>[3x]MAHHHHHHMSHCLIAPSIL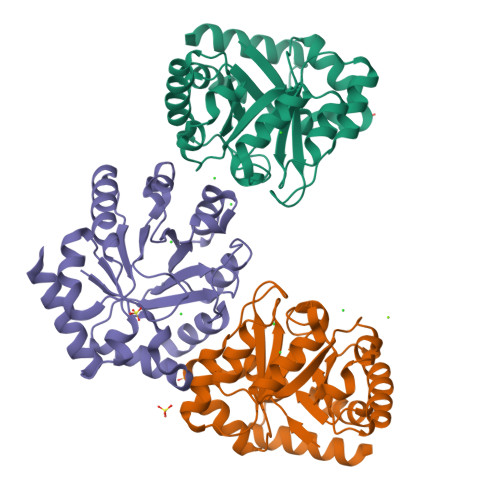SANFARLGEEVDNVLAAGADWVHFDVMDNHYVPNLTIGPMVCQALRKHGVTAPIDVHLMVEPVDRIIPDFAEAGATYISFHPEASRHVHRTIQLIRSLGCKPGIVLNPATPVDILDWVLDDLDLVLLMSVNPGFGGQAFIPSALDKLKVVRKMIDASGKDIRLEIDGGVKADNIGEIAAAGADTFVAGSAIFNAKTSYQDVIAQMRANVAAAR>[2x]MKWMCSICCAAVLLAGGAAQAEAVPNEPINWGFKRSVNHQPPDAGKQLNSLIEKYDAFYLGNTKEKTIYLTFDNGYENGYTPKVLDVLKK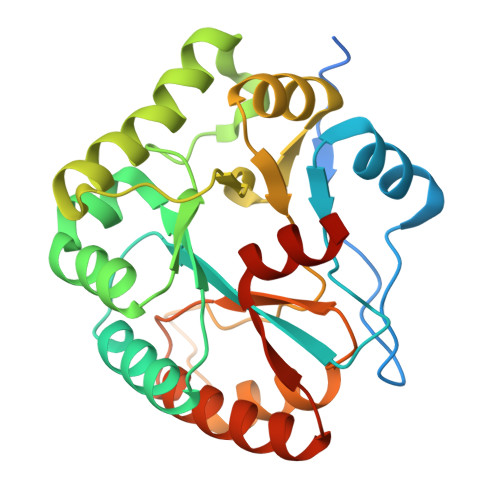HRVTGTFFVTGHFVKDQPQLIKRMSDEGHIIGNHSFHHPDLTTKTADQIQDELDSVNEEVYKITGKQDNLYLRPPRGVFSEYVLKETKRLGYQTVFWSVAFVDWKINNQKGKKYAYDHMIKQAHPGAIYLLHTVSRDNAEALDDAITDLKKQGYTFKSIDDLMFEKEMRLPSL In this report we identified that aaNAT5b is a SAT enzyme in the yellow fever mosquito Ae. aegypti. Although aaNAT5b recombinant protein displayed SAT activity to all tested substrates, spermine and agmatine are much better substrates than others. Although aaNAT5b shares only 8% sequence identity with human SAT, they have similar biochemical function, i.e. both acetylate spermine. Structurally, they both have motifs A and B, which are characteristics of N-acyltransferase superfamily proteins and an acetyl-CoA binding sequence folding similar for the cofactor binding.

In an effort to investigate the structure-function relationship of mosquito SAT enzyme and the substrate selectivity, efforts were made to crystallize its native enzyme and to soak them with its substrates or substrate analogues to determine its complex structure. After extensive optimizations, X-ray diffraction data was collected from the crystal of aaNAT5b soaked with hydrazine. The overall architecture of the structure is the same as in our previous report, with RMSD values of 0.1 to 0.5 Å between chains. However, a disulphide bond between residue 183 and residue 213 was found in the structure and it links two β strands (β7 and β6). In addition, residues 1–5 were modeled in the new complex structure, whereas they were not modeled in the previously reported structure because of the poor electron density in the region. All the test molecules are docked in the active center. Spermine interacts with Asp166, Val129, His130, Ser52, Asp48, Tyr28, Glu32 and Thr168 by hydrongen bonding and Tyr29, Phe51, Ile34, Trp101, Leu108, Val129, Ile131, Leu132, Gly165, Phe167, and Ser172 with hydrophobic interactions. Agmatine, spermidine, histamine, hexamethylenediamine, and putrescine share similar binding residues with spimine, but the enzyme has less interacting residues with them. Human SAT forms a dimer and the mosquito SAT is a monomer; mosquito SAT has a disulphide bond, and human SAT does not; and the conformation around the substrate binding sites is different between mosquito (two helixes) and human (one β strand), which may explain the substrate specificity of the individual enzymes.

>[2x]MVAPESIVLRVARLDELEQVREILHRIYYPEEGITISYVHGKSHTLDDERFSLSFVEQGTVVVAEDSAAKKFIGVSIAGPIQPGDPDAMVEEAATTETKKWGDILKLLALLERTADVCGRYGLEKAYHVHILAVDPTYRGHSLGQRLLQFQMDLSKKLGFKAISGDFTSVFSVKLAEKLGMECISQLALGDYRDEKGEKLFEPLDVHQVIKTCVKLL> STQNLGNSLMRVFSKEATRKYYLDLFKRADFTANLPKLAKKGGPDRLNDALKKLRKAGISEEKFAELKGAAA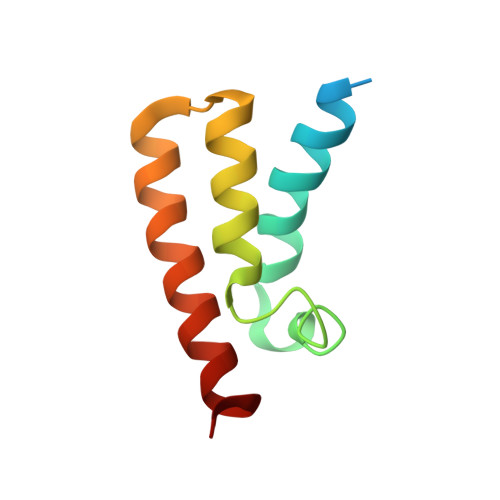KYADDWYRIYGK> VPGLLEDITR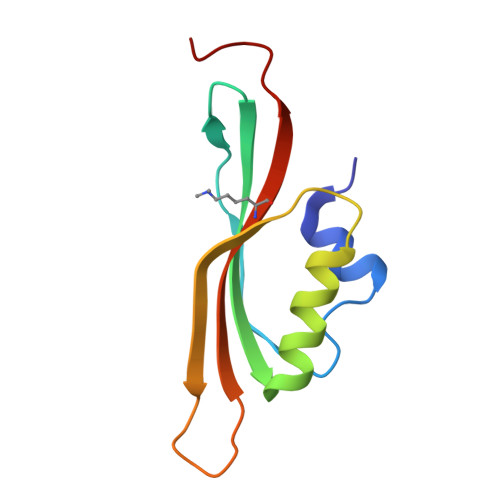TGLGSGLEFEEIKLLPEVAQQFYIELPIQISVVGGYHDLATFVSGVSSLPRIVTLHDFEIKPVAPGSTSKLRMSILAKTYRYNDKGLK> KKILIVDDEKPISDIIKFNM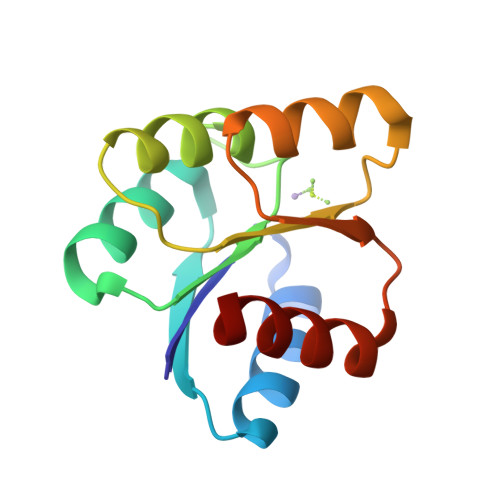TKEGYEVVTAFNGREALEQFEAEQPDIIILDLMLPEIDGLEVAKTIRKTSSVPILMLSAKDSEFDKVIGLELGADDYVTKPFSNRELQARVKALLRR>MSIEKIWAREILDSRGNPTVEVDLYTAKGLFRAAVPSGASTGIYEALELRDGDKQRYLGKGVLKAVDHINSTIAPALISSGLSVVEQEKLDNLMLELDGTENKSKFGANAILGVSLAVCKAGAAERELPLYRHIAQLAGNSDLILPVPAFNVINGGSHAGNKLAMQEFMILPVGAESFRDAMRLGAEVYHTLKGVIKDKYGKDATNVGDEGGFAPNILENSEALELVKEAIDKAGYTEKIVIGMDVAASEFYRDGKYDLDFKSPTDPSRYITGDQLGALYQDFVRDYPVVSIEDPFDQDDWAAWS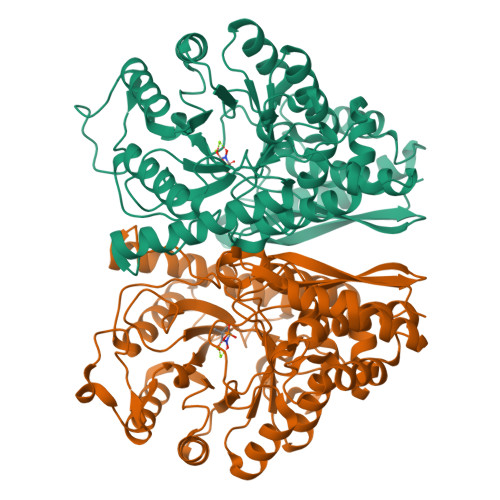KFTANVGIQIVGDDLTVTNPKRIERAVEEKACNCLLLKVNQIGSVTEAIQACKLAQENGWGVMVSHRSGETEDTFIADLVVGLCTGQIKTGAPCRSERLAKYNQLMRIEEELGDEARFAGHNFRNPSVLHHHHHH[8x]> EDSLTKQPEEVFDVLEKLGEGSYGSVFKAIHKESGQVVAIKQVPVESDLQEIIKEISIMQQCDSPYVVKYYGSYFKNTDLWIVMEYCGAGSVSDIIRLRNKTLIEDEIATILKSTLKGLEYLHFMRKIHRNIKAGNILLNTEGHAKLADFGVAGQLTDTMAKRNTVIGTPFWMAPEVIQEIGYNCVADIWSLGITSIEMAEGKPPYADIHPMRAIFMIPTNPPPTFRKPELWSDDFTDFVKK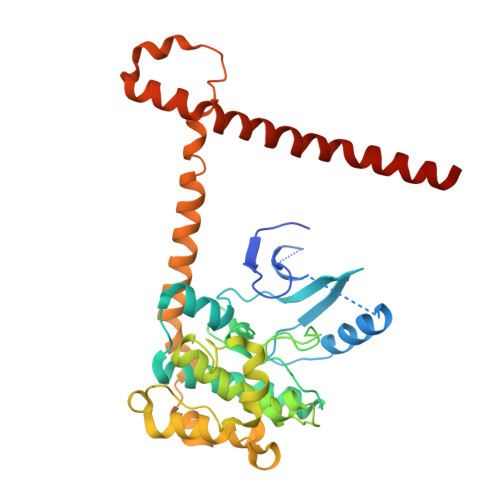CLVKNPEQRATATQLLQHPFIKNAKPVSILRDLITEAMEIKAKRHEEQQRELEEEENWKVPQDGDFDFLKNLSLEELQMRLKALDPMMEREIEELRQRYTAKRQPILDAMDAKKRRQQNF In Gram‐negative species, these bonds are introduced by the Dsb enzyme family, with DsbA acting as the primary thiol oxidase. B. pertussis' single DsbA (BperDsbA) (Heras et al., 2009) and DsbC (BperDsbC) enzymes have been shown to be essential for both the formation and stabilization of the pertussis toxin (PTX), a major virulence factor in B. pertussis infection (Scanlon et al., 2019; Stenson & Weiss, 2002). Notably, it contains a highly destabilizing catalytic Dsb, resulting in one of the most oxidizing redox potentials recorded for a DsbA enzyme. Functionally, BperDsbA shows limited substrate promiscuity and selectively catalyzes the oxidative folding of a pertussis toxin‐derived peptide, supporting a model of substrate specialization.

The structure of BperDsbA was solved to a resolution of 1.65 Å using molecular replacement and refined to R‐factor and R‐free values of 16.87% and 20.16%, respectively. The asymmetric unit contains two symmetrically independent monomers, both encompassing residues 1–179, which superimpose with a root‐mean‐square deviation (RMSD) of 0.432 Å across 179 equivalent Cα atoms. BperDsbA shares the canonical DsbA‐like architecture (Martin et al., 1993) with a TRX‐like core fold defined by the conserved motifs β₂α₁β₃ (residues 19–63) and β₄β₅α₇ (residues 130–179) separated by an alpha helical insertion domain. This insertion includes a three‐helix bundle (α₂, α₃, α₄; residues 64–111) and two additional helices (α₅ and α₆; residues 112–129). The active site includes conserved catalytic residues, with the CXXC motif (C28P29H30C31) located at the tip of α₁ (Quan et al., 2007) and the proline loop (G142T143P144) bridging α6 and β4 (inset) (Ren et al., 2009). Although the protein was oxidized prior to crystallization, the structure revealed BperDsbA in a reduced form, likely due to radiation damage. In this reduced state, hydrogen‐bond contacts were observed between the sulfur atom of Cys28 and the main‐chain nitrogen atoms of Pro29, His30, and Cys31 within the CPHC motif. Additionally, Cys28 forms hydrogen bonds with both the main‐chain carbonyl and side‐chain hydroxyl group of Thr144, a residue located in the cis‐proline loop (G142T143P144). Furthermore, BperDsbA exhibits an unusual surface electrostatic distribution, characterized by a positive patch directly above the active site and a negatively charged groove below. BperDsbA also exhibits notable structural differences compared to class Ia DsbAs such as EcDsbA, including a restructured β5–α7 loop that produces a narrower peptide‐binding groove more consistent with class Ib DsbAs (McMahon et al., 2014; Santos‐Martin et al., 2021) and distinct surface electrostatics.

>[2x]QQYVNINPPMPSDTPGKIEVLEFFAYTCPHCAAIEPMVEDWAKTAPQDVVLKQVPIAFNAGMKPLQQLYYTLQALERPDLHPKVFTAIHTERKRLFDKKAMGEWAASQGVDRAKFDSVFDSFSVQTQVQHASQLAEAAHIDGTPAFAVGGRYMTSPVLAGNDYAGALKVVDQLIVQSRK(2R,5S,11R,14R)-5,8,11-trihydroxy-2-(nonanoyloxy)-5,11-dioxido-16-oxo-14-[(propanoyloxy)methyl]-4,6,10,12,15-pentaoxa-5,11-diphosphanonadec-1-yl undecanoate | 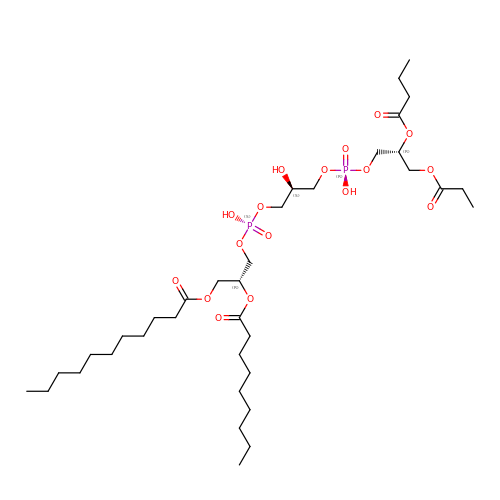C36 H68 O17 P2 | FMNZIMGRZPIVKW-XWHIBYANSA-N>SNAMSYRNKTYVAFASEDIKFYRLMEAWKANEKIDFNFFDAHDLFISRDTSKPETIKRNLRERMKNAKQVVLLGSGNTKRKGSDGVSFLAHEIDLIVEFNLPVVIANLDGDRTVDKNFIPKPLLDSEHYTVSVSFQPKIIKYALDNYCVNYYSSSNSGSYLYPTSVYTKLGL[3x]

The Thoeris defense system triggers abortive infection (Abi) upon phage detection. The ThsB genes encode Toll/interleukin-1 receptor (TIR) domain–containing proteins responsible for phage detection, while the ThsA gene encodes an Abi-triggering effector protein. Two ThsA effector variants have been reported: a silent information regulator (SIR2) and SMF/DprA-LOG (SLOG) domain–containing effector (ThsASIR2-SLOG) and a transmembrane (TM) and macro domain–containing effector protein (ThsATM-macro). Collectively, our biochemical and structural data demonstrate that the nucleotide signaling requirements for ThsASIR2-SLOG and ThsATM-macro effectors are distinct and suggest that ThsATM-macro effectors can trigger Abi via membrane perturbation by a mechanism that involves nucleotide-induced oligomerization of its macro domain.

The Thoeris defense system in E. coli CFT073 consists of a TM-macro ThsA effector (EcThsA) and two TIR domain–containing ThsB proteins (EcThsB1 and EcThsB2). To identify the nucleotide products generated by ThsB proteins of Thoeris systems with a TM-macro ThsA effector, we expressed and purified the TIR domains of EcThsB1 (EcThsB1TIR) and EcThsB2. We did not detect NADase activity for EcThsB2, but its crystal structure revealed a unique active site configuration with a tyrosine residue within hydrogen bonding distance to the catalytic glutamate residue. Furthermore, AlphaFold2 modeling reveal that many ThsB proteins (subfamilies 7 to 9) found in Thoeris systems with a ThsATM-macro effector have an active site configuration closely related to the NDT family of enzymes, which catalyze base-exchange reactions between the purine or pyrimidine bases of 2′-deoxyribonucleosides and free pyrimidine or purine bases. Our structural data suggest that EcThsB2 may be autoregulated, in this case, by a short C-terminal extension that binds to a surface region shown to be important for TIR domain self-association and active site formation in SARM1 and AbTir. To test whether this tail affects ThsB activation, we generated two variants of EcThsB2: a modified tail with Y159 and Y164 replaced by alanines (EcThsB2Y159A, Y164A) and a tail deletion (EcThsB2Δ151–169). However, neither of the variants could be expressed in a soluble form in E. coli, suggesting that this tail may also be required for proper folding of EcThsB2. Together, these structural analyses identify a class of TIR domains with a unique active site configuration associated with TM-macro Thoeris systems. The single ThsB protein of BaThs has a tyrosine containing active site and a predicted structure (UniProt/AlphaFold Database: A0A806QQ11) similar to EcThsB2 and ThsB subfamily 9 members, suggesting that this class of ThsB proteins produces histidine adenine dinucleotide as an immune signaling molecule.>[4x]MGSSHHHHHHSSGENLYFQGHMTLSITSNFDAGAIDVVSCDSPDAIRLRVRGDNRSEFAQWFYYRLTGARGERCVMTFENAAECAYPSGWRNYSAVASYDRVDWFRVPTTFDGKTMTIDHTPEFDSIYYAYFEPYSEERHAAFLGAVQQLPQASVVELGRTVEGRPMSLLTLGTPETDGAPKKKV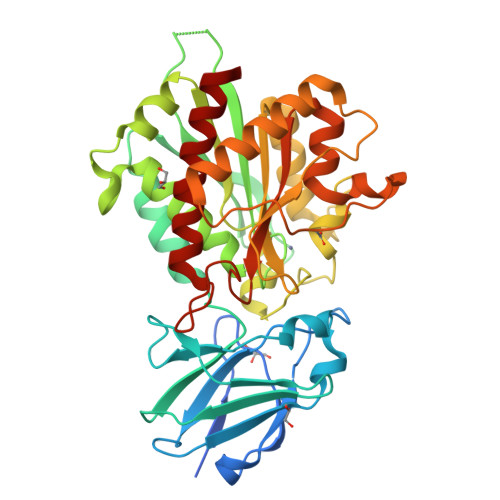WIIARQHPGESMAEWFVEGLVKRLAGWGDWAGDPVARKLYDRVTFHIVPNMNPDGSVHGNLRTNAAGANLNREWMAPDAERSPEVLAVRDAIHAIGCDMFFDIHGDEDLPYVFVAGSEMLPSFTEQQGKEQTAFIEAFKVASPDFQTEHGYAASKYKEDALKLASKYIGHQFGCLSLTLEMPFKDNANLPDERVGWNGERSAALGAAMLAAILVHVDTFA>[2x]GPLGSRRKFMEFPYVSPTRKQLMVDLMSTVENRLQSQLLPCNLPPDVRNFNNPNGSAEASLHIRSGDKSSPIDFVIGSWIHCKIPTGVSLNITSISGFLNSSTKAPNFVVELIQSSSKSLVLILDLPHRKDLVLNPDYLKEYYQDTALDSHRQSLLKLPEVNPYVSPSLFVRSAFSPTASMLKIDAEEEDKLEEIL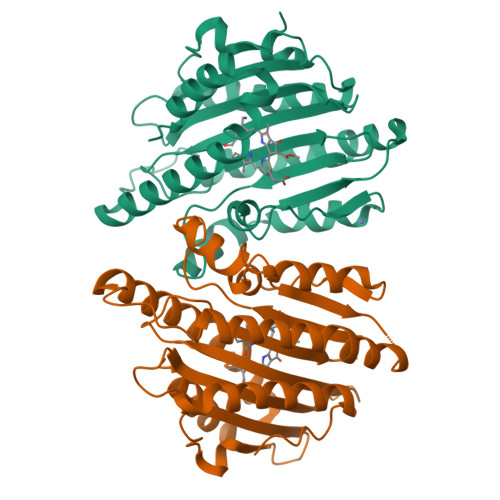RDHVSPAAKEVLEVWLERCVKEEEEKIVVGEEERMELERRDKSFRRKSIEDDLDLQFPRMFGEEVSSRVVHAIKEAFGVL>MSTRKAVIGYYFIPTNQINNYTETDTSVVPFPVSNITPAKAKQLTHINFSFLDINSNLECAWDPATNDAKARDVVNRLTALKAHNPSLRIMFSIGGWYYSNDLGVSHANYVNAVKTPASRAKFAQSCVRIMKDYGFDGVDINWEYPQAAEVDGFIAALQEIRTLLNQQTITDGRQALPYQLTIAGAGGAFFLSRYYSKLAQIVAPLDYINLMTYDLAGPWEKVTNHQAALFGDAAGPTFYNALREANLGWSWEELTRAFPSPFSLTVDAAVQQHLMMEGVPSAKIVMGVPFYGRAFKGVSGGNGGQYSSHSTPGEDP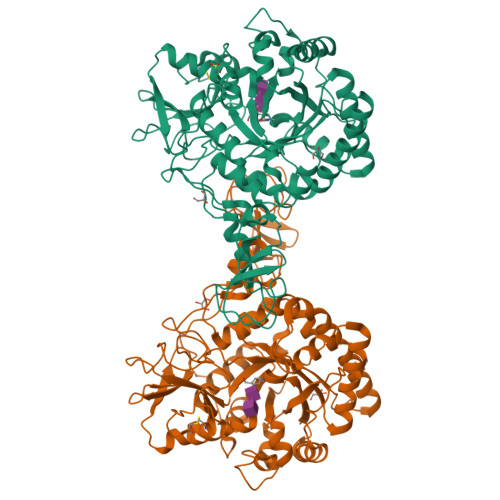YPSTDYWLVGCEECVRDKDPRIASYRQLEQMLQGNYGYQRLWNDKTKTPYLYHAQNGLFVTYDDAESFKYKAKYIKQQQLGGVMFWHLGQDNRNGDLLAALDRYFNAADYDDSQLDMGTGLRYTGVGPGNLPIMTAPAYVPGTTYAQGALVSYQGYVWQTKWGYITSAPGSDSAWLKVGRVA[2x]> GSMKKVEAIIRPEKLEIVKKALSDAGYVGMTVSEVKGRGVQGG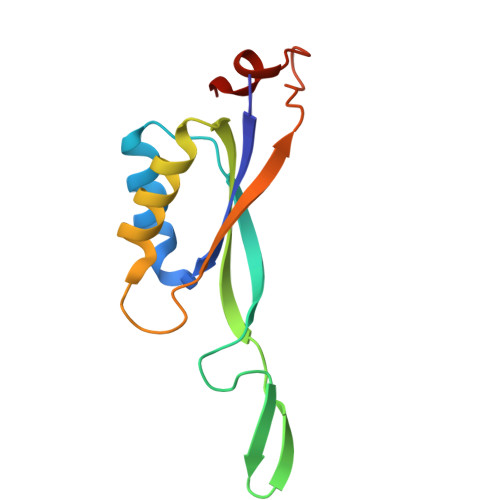IVERYRGREYIVDLIPKVKIELVVKEEDVDNVIDIICENARTGNPGDGKIFVIPVERVVRVRTKEEGKEALEEHHH2-AMINOTHIAZOLINE | C3 H6 N2 S 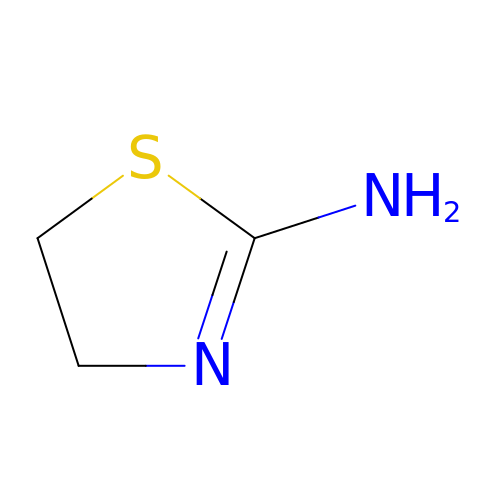| REGFWZVTTFGQOJ-UHFFFAOYSA-N> DMPVERILEAELAVEPKTETYVEANMGLNPSSPNDPVTNICQAADKQLFTLVEWAKRIPHFSELPLDDQVILLRAGWNELLIASFSHRSIAVKDGILLATGLHVH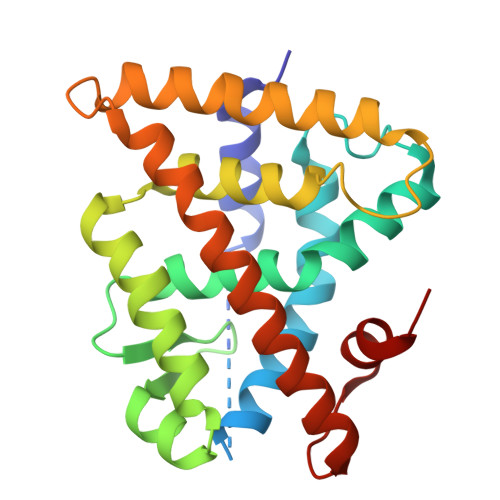RNSAHSAGVGAIFDRVLTELVSKMRDMQMDKTELGCLRAIVLFNPDSKGLSNPAEVEALREKVYASLEAYCKHKYPEQPGRFAKLLLRLPALRSIGLKCLEHLFFFKLIGDTPIDTFLMEMLEAP>MKKLGTLLVLFLSAIILVACASGKKDTTSGQKLKVVATNSIIADITKNIAGDKIDLHSIVPIGQDPHEYEPLPEDVKKTSEADLIFYN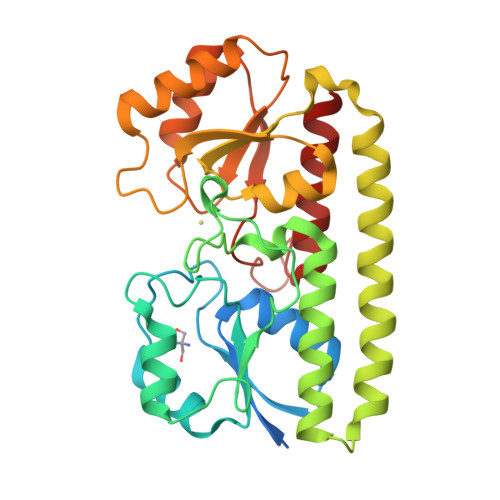GINLETGGNAWFTKLVENAKKTENKDYFAVSDGVDVIYLEGQNEKGKEDPHAWLNLENGIIFAKNIAKQLSAKDPNNKEFYEKNLKEYTDKLDKLDKESKDKFNKIPAEKKLIVTSEGAFKYFSKAYGVPSAYIWEINTEEEGTPEQIKTLVEKLRQTKVPSLFVESSVDDRPMKTVSQDTNIPIYAQIFTNSIAEQGKEGDSYYSMMKYNLDKIAEGLAK[2x]2'-deoxy-5-[(4-ethynylphenyl)ethynyl]uridine 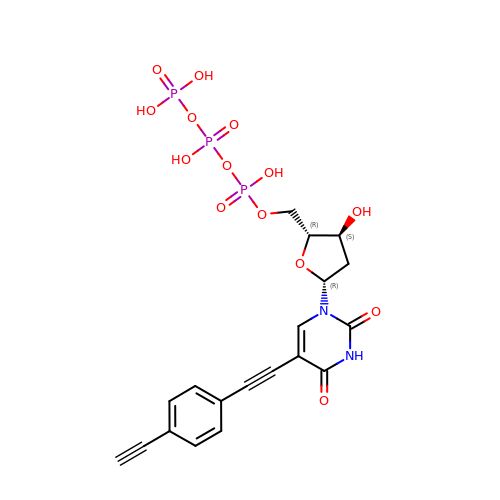5'-(tetrahydrogen triphosphate) | C19 H19 N2 O14 P3 | NDHYKBWELLKQHS-GVDBMIGSSA-N> MRGSHHHHHHGSMPVAGSELPRRPLPPAAQERDAEPRPPHGELQYLGQIQHILRCGVRADDRTGTGTLSVFGMQARYSLRDEFPLLTTKRVFWKGVLEELLWFIKGSTNAKELSSKGVKIWDANGSRDFLDSLG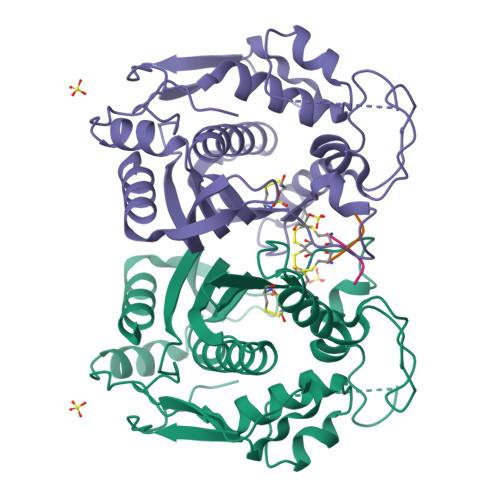FSTREEGDLGPVYGFQWRHFGAEYRDMESDYSGQGVDQLQRVIDTIKTNPDDRRIIMCAWNPRDLPLMALPPCHALCQFYVVNSELSCQLYQRSGDMGLGVPFNIASYALLTYMIAHITGLKPGDFIHTLGDAHIYLNHIEPLKIQLQREPRPFPKLRILRKVEKIDDFKAEDFQIEGYNPHPTIKMEMAV;> CQLY>[6x]MASWSHPQFEKIEGREPLHLPILEFKTEYRYPSTFEHEAQFKDTVLEFLAHEASDIIIKQGVAISAKVKGTLCTLSTRTLNFNEIERIALWASGSSSVLTELASKKLINTRYEVFHPTKLTTGGQKQRFGYRVNISPVYIQGKTTAEIVMRSIPLDPLPLADIGLSPELVNQMCPDNGIVMVAGKTSSGKSTTFSSIIRYIMENDTPIKGHLLTHEDPIEFVYDNIKSAHSIIAQSQIPEQFSSFAIANQEALRRTPNLIMIGELRDKQSIESAFEAANTGHPVFATVHSQNCSAVMRRLISRFDESVRGAAIYDLVETTRFIMAQTLVRKTDGNLVAAREYLNFTTDIREQLLSLSDMGKVASEVRRLVDEFGHPFSLEAERLHSDGIIDGHVAKRLSMMS

The dot/icm T4bS system of L. pneumophila is powered by two ATPases: The membrane protein DotL, which is part of the coupling sub‐complex responsible for the recruitment of substrates and their delivery to the secretion channel and DotB, potentially involved in complex assembly and secretion. Here we present the X‐ray crystal structures of two DotB proteins, one from the dot/icm system encoded by the L. pneumophila genome (termed DotBL), at 3.19 Å resolution, and one from the dot/icm system encoded in the plasmid of Y. pseudotuberculosis IP31758 (termed DotBY), at 2.75 Å resolution. DotBL and DotBY subunits display a very similar topology. A DotBL or Y subunit is composed of a ∼150 aminoacids long N‐terminal domain (NTD), comprising 6 β‐strands and 3 α‐helices, and a ∼250 aminoacids C‐terminal domain (CTD) consisting of 7 β‐strands and 10 α‐helices [Fig. 1(A,B)]. The main part of the CTD adopts a RecA fold and harbours the signature motifs of the AAA+ family: The Walker A motif between β7 and α5 (also referred as P‐loop), the Asp Box on β8, the Walker B motif on β10 and the His Box on β11.

Homologs of the dot/icm system are found in most Legionella species, but also in other pathogens, such as Coxiella burnetii responsible for Q‐fever, or Yersinia pseudotuberculosis strain IP31758, responsible for the Far East Scarlet‐like fever. The DotBY hexamer differs from the DotBL hexamer in exhibiting an ααβααβ arrangement instead of the αβαβαβ arrangement observed in DotBL. In DotBY, A, B, D, and E are in the α conformation, while C and F are in the β one, yielding an overall twofold symmetry. Interestingly, the two DotB proteins we have investigated have different hexameric organization, with DotBL consisting of trimer of α–β dimers, whereas DotBY consists of dimers of α–α–β trimers. The DotBY protein was crystallized without any phosphate or nucleotide in the buffer. Nevertheless, when analyzing the ATP‐binding site region of all six subunits, we observed a striking difference between chains adopting the α and β conformations [Fig. 4(F)]. In the β conformation (chains C and F), the Walker A region is similar to what is observed in the bound structures of DotBL and other ATPases, namely we observe an unwinding of the first α‐helical turn of α5 rich in Ser/Gly that provides space for a phosphate to bind. Surprisingly, in the α conformation of DotBy (chains A, B, D, and E), this α‐helical turn is present, formed with the carboxyl groups of residues Ser173 and Ser174 (equivalent to Ser159 and Gly160 in DotBL) contacting the NH groups of Ser177 and Thr178 respectively. With such configuration, a phosphate group would not have the space to bind at this position. Interestingly, in the structures of PilT, PilT2, PilB, EpsE, and VirB11, this additional α‐helical turn of the P‐loop is not observed.>[2x]GFKQDIATLRGDLRTYAQDIWLAFLNKYPDEKRNFKNYVGKSDQELKSMAK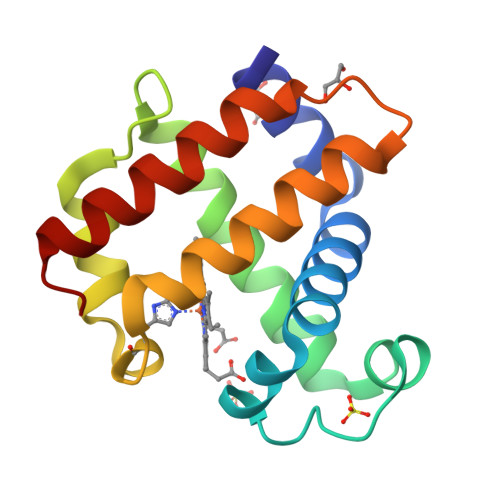FGDHTEKVFNLMMEVADRATDCVPLASDASTLVQMKQHSGLTTGNFEKLFVALVEYMRASGQSFDSQSWDRFGKNLVSALSSAGMK>GMGQDKLKVAVLFGGSSEERDVSIASGAQVIQALRSAGHQVLAVDTASGLLGAEEERRLLASKVKEVPPDSDSLAIIRSGKQSLLSAGELAGVDVFFLALHGGTGEDGTLQALLDAGGFAYTGSGHLASAMAMDKDVAKRLFLAAGVETASWLMAPASEEEVREQLGFPLVVKPNSQGSTVGLSIVHSQAELQPAIELAGRYGDEVMLERFVAGREVTVGVLDDQALPVGEILLGGQEVFDYEHKYQAGAVREVFPADLPPAIAAEAQRLALKVHRALKLSGYSRTDFRLDEQGRLWCLEVNTLPGMTATSLLPQAAAAAGIGFAELCERICRLGIERCKGAR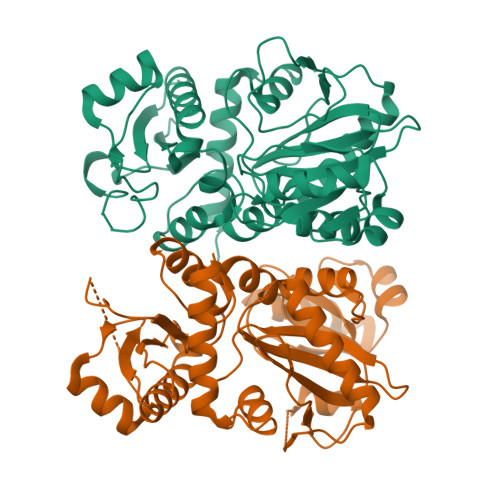KARS[4x]3-[6-(oxan-4-yl)pyridin-2-yl]phenol 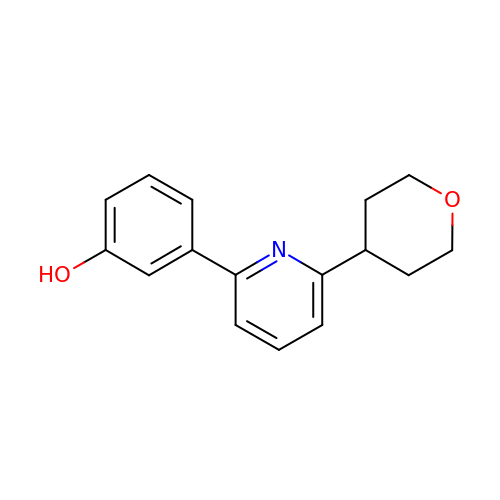| C16 H17 N O2 | JWOOVEVAKYLUGG-UHFFFAOYSA-N> GSPTFKSAVKALFDYKAQREDELTFTKSAIIQNVEKQDGGW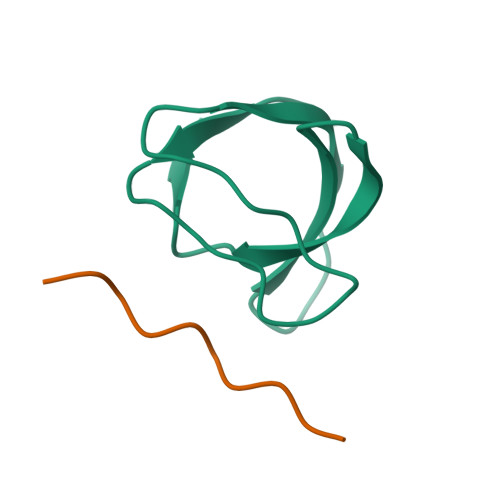WRGDYGGKKQLWFPSNYVEEMIN;> QPPVPPQRPM>[2x]ATKIDKEAC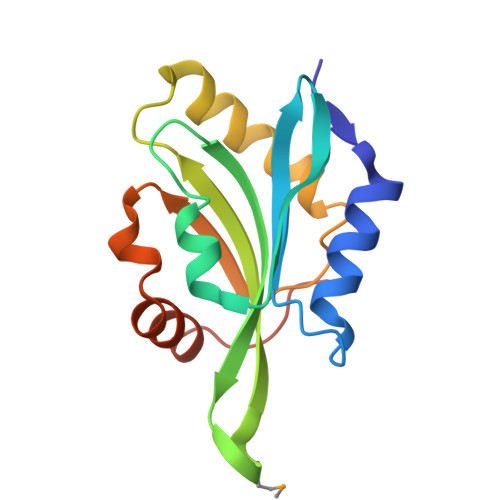RAAYNLVRDDGSAVIWVTFKYDGSTIVPGEQGAEYQHFIQQCTDDVRLFAFVRFTTGDAMSKRSKFALITWIGENVSGLQRAKTGTDKTLVKEVVQNFAKEFVISDRKELEEDFIKSELKKAGGANYDAQTE>SANEDMPVERILEAELAVEPKTETYVEANMGLNPSSPNDPVTNICQAADKQLFTLVEWAKRIPHFSELPLDDQVILLRAGWNELLIASFSHRSIAVKDGILLATGLHVHRNSAHSAGVGAIFDRVLTELVSKMRDMQMDKTELGCLRAIVLFNPDSKGLSNPAEVEALREKVYASLEAYCKHKYPEQPGRFAKLLLRLPALRSIGLKCLEHLFFFKLIGDTPID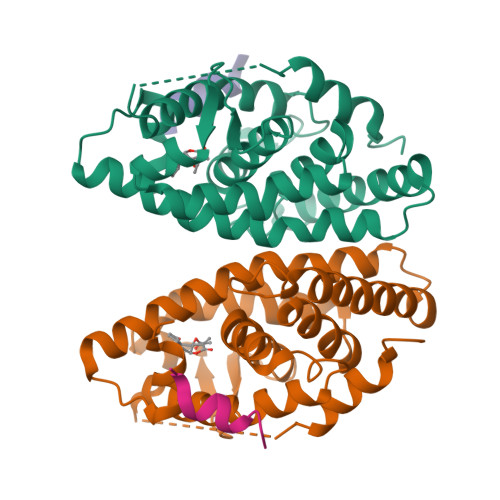TFLMEMLEAPHQMT[2x];>KHKILHRLLQD[2x]>GAMNPLAQSLNEQLQQSNATAFAMLSDLGQNMFYPKGILSQSAEAKSTTYNATIGMATNKDGKMFASSLDAMFNDLTPDEIFPYAPPQGIEELRDLWQQKMLRDNPELSIDNMSRPIVTNALTHGLSLVGDLFVNQDDTILLPEHNWGNYKLVFNTRNGANLQTYPIFDKDGHYTTDSLVEALQSYNKDKVIMILNYPNNPTGYTPTHKEVTTIVEAIKALANKGTKVIAVVDDAYYGLFYEDVYTQSLFTALTNLHSNAILPIRLDGATKEFFAWGFRVGFMTFGTSDQTTKEVLEAKVKGLIRSNISSGPLPTQSAVKHVLKNNKQFDKEIEQNIQTLKE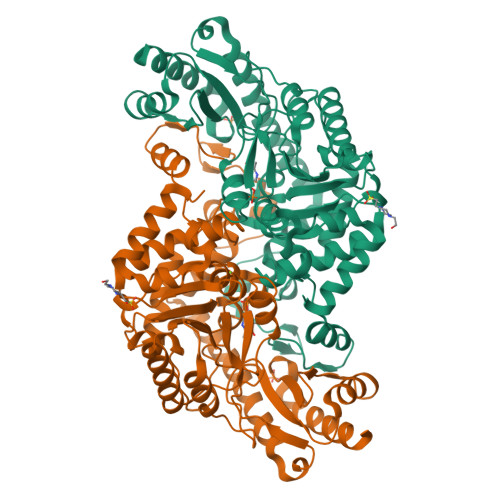RYEVTKEVVYADQYHSHWQAYDFNSGYFMAIKVHDVDPEALRKHLIDKYSIGVIALNATDIRIAFSCVEKDDIPHVFDSIAKAIDDLR[2x]>[3x]MLEARLEQASLLKRVVDAIKDLVQDCNFDCNDSGIALQAMDNSHVALVSMLLKAEGFSPYRCDRNIALGINLVSLTKVLRAAQNEDILTLKADDSPDAVNLMFESAETDRISEYDIKLMDIDQEHLAIPETEYAATVEMPSAEFQRICRDLNALSESVVIE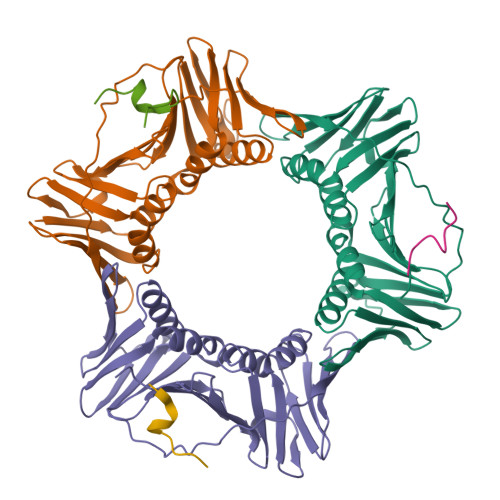ATKEGVKFSCQGDIGSGSVTIRQHTSVDKPEQNVSIALSEPVALTFSLKYLVNFCKATSLSSKVTLCLSQEVPLLVEYGLGSGHLRFYLAPKIGDE;>KRRMPTDIRNFFHSKR[3x]> YFGGLNAQYQTDITTLAKGISNAGLKMEYILFDDCYMSSIEVAYALKDVTDYLIGSTSEVMAYGMPYAEIGQYLIGKVDYAGICDGFYSFYSTYSTPCGTIAVTDCSELDNLATIMKEINHRYTFDPSLTSSL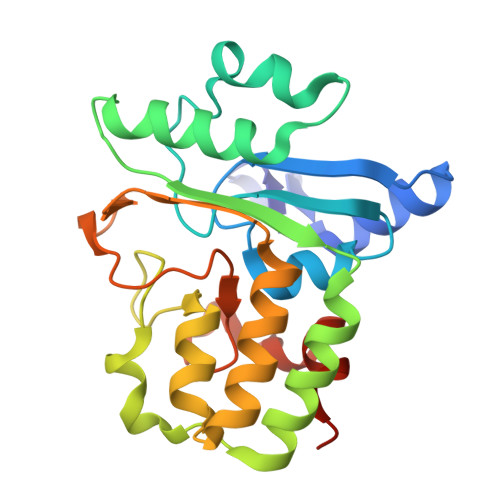QRLDGYYPVIFFDYGDYVSKLCPDETLVARFNEQLNRTVPFKRNTEYFYSMSRGEVKINTFSGITISDPSTHSLASKKEETAWYAATHLEHHHHHH> MAKKTSSKGKLPPRVPNLIPYVGSFVSFAKNPVQFIIDNSKKYGDVFTATILGKEMTFLNHPKILDTFFKATDNELSLRDVYRFMRPVFGTGVVYDADSTERMMEQVKFVSSGLTTARFRVFVDIFEDEIAHKVKELGPEGTVDVAELMADLIIFTASRCLLGDEVRQYLSEKNLGKLYHDIDDGISPLSFFYPSLPAPKRDKARKAVGEIFQELLDKRREEHKKHPERLLDESKMDVVDHLLTQKYKDGQELTDVHRIGILIAGLFAGQHTSSITSSWTLMNVISNKKVLEKVRKEQEEIMGSDKVLDYDKVMKMDYLEACMKEALRMYPPLIMIMRMARKPRECEQYIIPKGNILVVSPSVAGRCTDTYTNPDVFDPERLTERKEHEKFKYGAVPFGAGRHKCIGENFALLQVKSIISILLRYFDMEYIGKIPDPSYTSLVVGPSPPTRMRYKLRKQQHHHHHH

We used a combination of cheminformatics, target-, and phenotypic-based drug discovery methods to identify inhibitors that target an essential N. fowleri enzyme, sterol 14-demethylase (NfCYP51). The amoebicidal effect of CYP51 inhibitors is due to inhibition of 14-demethylation of the endogenous CYP51 substrate in N. fowleri, 31-norlanosterol. 14-Demethylation of 31-norlanosterol is a prerequisite for subsequent 4α-demethylation and 24-methylation steps, leading to biosynthesis of essential ergosterol and ergosterol-like sterols. Depletion of ergosterol, concomitant with the accumulation of intermediates and end-products incompatible with normal permeability and fluidity of the Naegleria cell membrane, leads to the altered morphology and death of N. fowleri cells.

The top hit (2a) had a miconazole-like scaffold (1) and was singled out following cocrystallization with the NfCYP51 target. Only one compound, 2a (used as a racemic mixture), produced cocrystals with the target. The well-defined electron density in the binding pocket adjacent to heme corresponds to the S-configuration at the chiral carbon center of 2a. Superimposition with fluconazole indicates that both molecules coordinate to the heme iron with the azole moiety, while other aromatic moieties of each compound are engaged in different sets of drug–target interactions. The cocrystal structure of 2a revealed three main groups of drug–target interactions. The aromatic nitrogen atom of the imidazole moiety provided a coordination bond to the heme iron. (b) The 3-trifluoromethyl-benzoyl moiety is somewhat coplanar to the heme plane. (c) Finally, the 4-fluorophenyl moiety projects toward the long hydrophobic tunnel extending from the heme to the protein surface known to accommodate large hydrophobic moieties in higher molecular weight azole inhibitors (posaconazole and itraconazole). The C2–C3 edge of the 4-fluorophenyl moiety faces heme propionate (6.3 Å) and the OH-groups of Tyr107 (5.3 Å) and Tyr120. For CNS compatibility, we propose staying within the binding envelope of 2a and avoiding extending molecules into the hydrophobic tunnel.3-{3-[(naphthalen-1-yl)oxy]propyl}-1H-indole-2-carboxylic 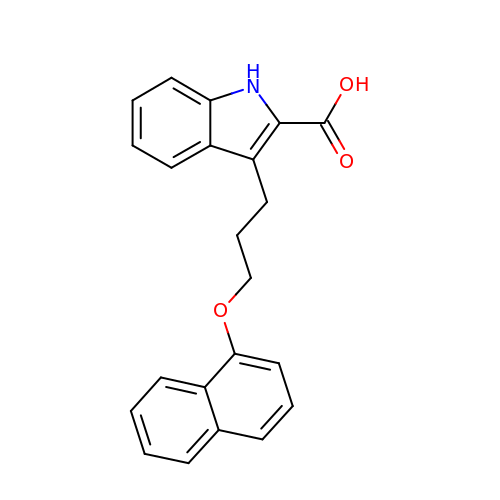acid | C22 H19 N O3 | IQTBMDSOBZUIII-UHFFFAOYSA-N>MGSSHHHHHHSQDPMPIAVGMIETLGFPAVVEAADAMVKAARVTLVGYEKIGSGRVTVIVRGDVSEVQASVSAGLDSAKRVAGGEVLSHHIIAR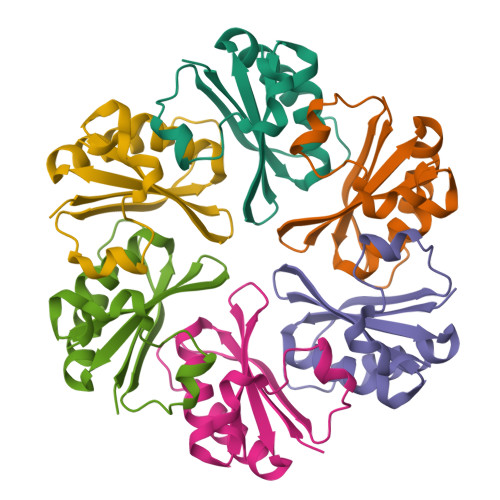PHENLEYVLPIRYTEAVEQFRM[6x]> ATIRYSVAEEMESGSFVANVAKDLGLEVGKLAERGARLVAEGNRLHFRLHRKTGDLFVKEKLDREALCGKSDPCVLHFEIILAEPLQSFRVEVRVFDINDNAPVFLNKEPLLKIPESTPLGSRFPLQSAQDLDVGLNG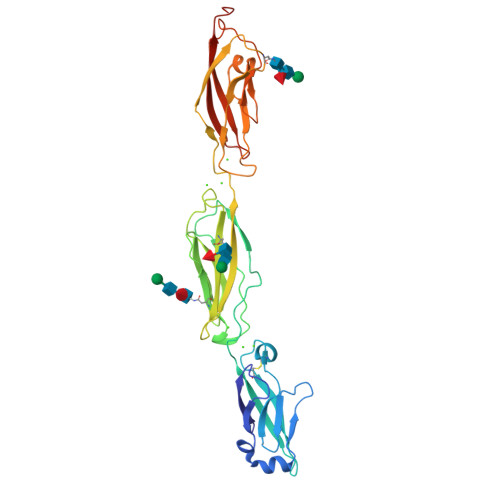LQNYTLSANTYFHLHTRFRSHGPKYAELVLDNPLDREAQPEVNLTITAVDGGSPPKSGTANIRVVVLDVNDHVPQFSRLVYRAQVPENSDNGSLVVVVTATDLDEGTNKQITYSLAENPEAVLRTFLVDPQTGEVRLRGPLDFEMIETYDIDIQATDGGGLSAHSKVLVEVVDVNDHHHHHHHH(5E)-5-(QUINOXALIN-6-YLMETHYLENE)-1,3-THIAZOLIDINE-2,4-DIONE | C12 H7 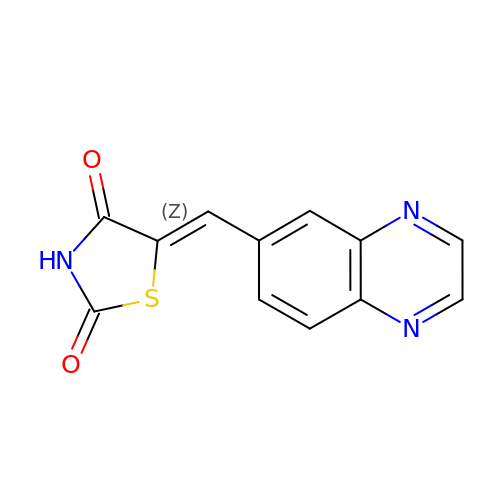N3 O2 S | SQWZFLMPDUSYGV-POHAHGRESA-N N-ALPHA-ACETYL-3,5-DIIODOTYROSYLGLYCINE | C13 H14 I2 N2 O5 | 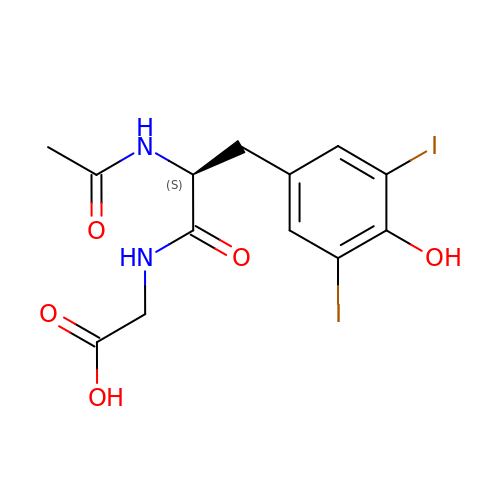SXRYVFRVDCDPKH-JTQLQIEISA-N>[2x]MSLSKVFTIGEILVEIMASKIGQPFDQPGIWNGPYPSGAPAIFIDQVTRLGVPCGIISCVGNDGFGDINIHR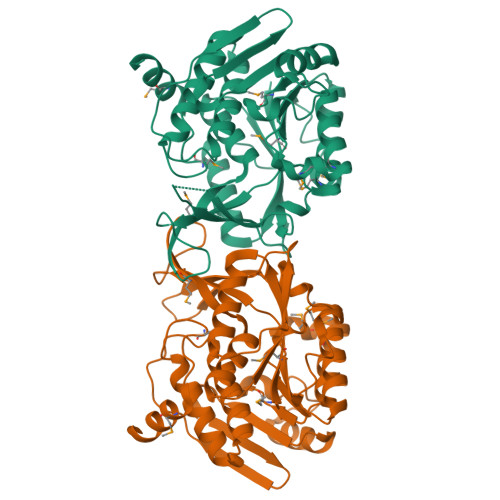LAADGVDIRGISVLPLEATGSAFVTYHNSGDRDFIFNIKNAACGKLSAQHVDENILKDCTHFHIMGSSLFSFHMVDAVKKAVTIVKANGGVISFDPNIRKEMLDIPEMRDALHFVLELTDIYMPSEGEVLLLSPHSTPERAIAGFLEEGVKEVIVKRGNQGASYYSANEQFHVESYPVEEVDPTGAGDCFGGAWIACRQLGFDAHRALQYANACGALAVTRRGPMEGTSRLMEIETFIQRHDMSIREAAQEGHHHHHH> GSINMATVPVYCVCRLPYDVTRFMIECDACKDWFHGSCVGVEEEEAPDIDIYHCPNCEKTHGKSTLKKKRTWHKHGPGQAPDVKPVQNGSQLFIKELRSRTFPSAEDVVARVPGSQLTLGYMEEHGFTEPILVPKKDGLGLAVPAPTFYVSDVENYVGPERSVDVTDVTKQKDCKMKLKEFVDYYYSTNRKRVLNVTNLEFSDTRMSSFVEPPDIVKKLSWVENYWPDDALLAKPKVTKYCLICVKDSYTDFHIDSGGASAWYHVLKGEKTFYLIRPASANISLYERWRSASNHSEMFFADQVDKCYKC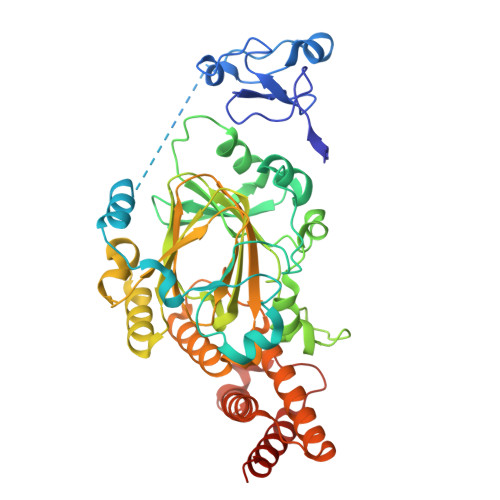IVKQGQTLFIPSGWIYATLTPVDCLAFAGHFLHSLSVEMQMRAYEVERRLKLGSLTQFPNFETACWYMGKHLLEAFKGSHKSGKQLPPHLVQGAKILNGAFRSWTKKQALAEHEDELPEHFKPSQLIKDLAKEIRLSENASKAVRP> ISEFDSEGSNMSTTAHTEPSWADLPFLDFTDPNFSWDSPEVAEAREKSWIARTPLALLVLRYAEADQLARDKRLISGFRGLVDMVGTPEGPVRDFMVDFLQSLDGADHRRLRGLATHPFTPRRITAVQPFVRSTVEQLIDKLPQGDFDFVQHFPHPLPALVMCQLLGFPLEDYDTVGRLSIETNLGLALSNDQDILVKVEQGLGRMFDYLVAAIEKRKVEPGDDLTSDIVRAFHDGVLDDYELRTLVATVLVAGYETTNHQLALAMYDFAQHPDQWMKIKENPELAPQAVEEVLRWSPTLPVTATRVAAEDFEVNGVRIPTGTPVFMCAHVAHRDPRVFADADRFDITVKREAPSIAFGGGPHFCLGTALARLELTEAVAALATRLDPPQIAGEITWRHELGVAGPDAL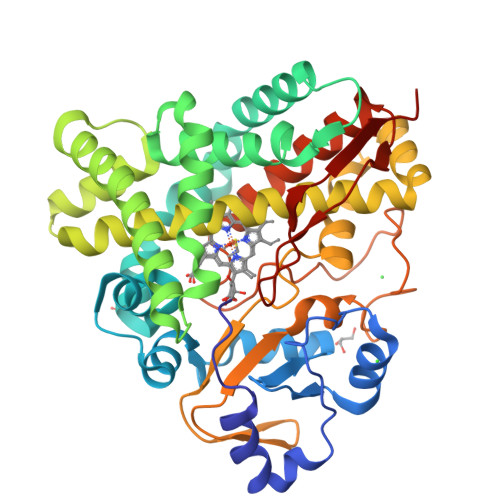PLRFGAA> DPMAEPASVAAESLAGSRARAARTVLGQVVLPGEELLLPEQEDAEGPGGAVERP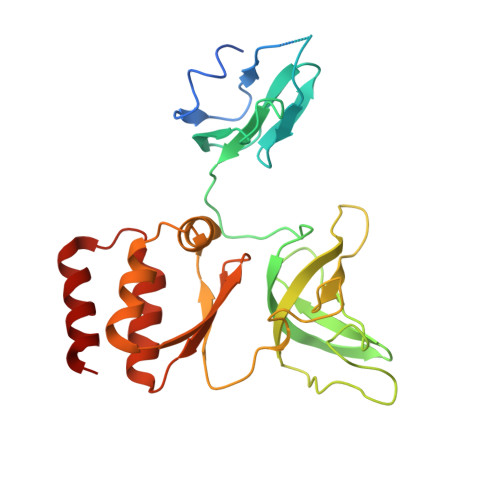LSLNARACSRVRVVCGPGLRRCGDRLLVTKCGRLRHKEPGSGSGGGVYWVDSQQKRYVPVKGDHVIGIVTAKSGDIFKVDVGGSEPASLSYLSFEGATKRNRPNVQVGDLIYGQFVVANKDMEPEMVCIDSCGRANGMGVIGQDGLLFKVTLGLIRKLLAPDCEIIQEVGKLHPLEIVFGMNGRIWVKAKTIQQTLILANILEACEHMTSDQRKQIFSRLAES> VRPNQGRNDYNQVGGKKRGQGVQVLPETIRLLIETRKAATAGGPVGRQPLPKATEATGVSSWGRDRRFPITEALRLPTVAEVNAPWEPYDETANKRRSGSRPLSSSVDGCHENHDPSSDGVARGQDRLGRLDKVVLHSGDISRLRVDATVVGAVRSFKTVGDGRGFTGCSALLEGAGPFLSSFVSQQRRHLGEELLHTPVRGDPSSAQTVAAAAVRGLRRGIHHFTASTVPLPLRSSSTVPSLAEVEEMPIMELSQLAARAALLGSARGGGTRGFGLSSHPQTRRLEGVSTASGATEGSDAALSFANEVRDQATASQFPARDLIQTPLDPSQLSPPGAVLISPGFNLPSNFLIHVAEPNAV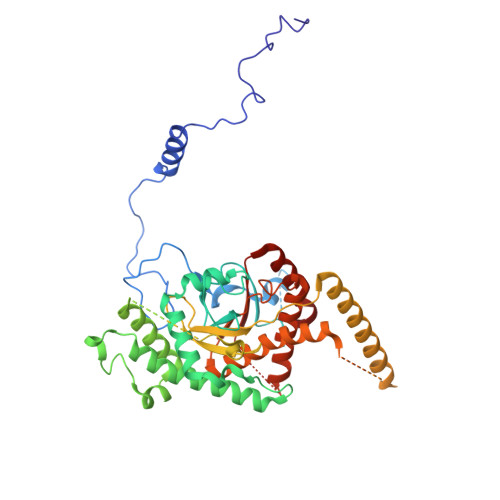LSNQQMLDTLFRLEEREALRRKEQLLSRFGAAQAADEAMSDDEVREEDNEMTPRSMWQDDAERDTGVQRMLLLEECYINALNAAWALGVRSVALPCLGAGVGRFPVYIAARCAARGVARWMSEHRDCDAWENAESDKRADFDRIVFCTSSDVEWNALRRVIPQFLS> SNIKSLSFPKL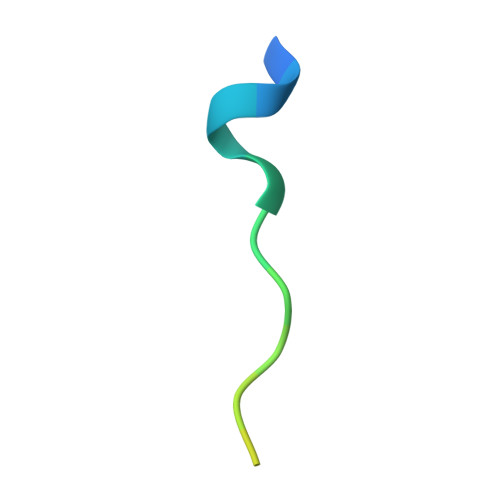DSDDSNQKT>MHHHHHHFNL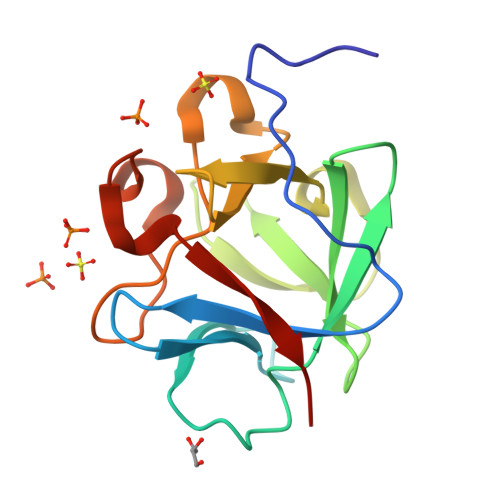PPGNYKKPKLLYCSNGGHFLRILPDGTVDGTRDRSDQHIQLQLSAESVGEVYIKSTETGQYLAMDTDGLLYGSQTPNEECLFLERLEENHYNTYISKKHAEKNWFVGLKKNGRCKRGPRTHYGQKAILFLPLPVSSD[2x]> MEVHDFETDEFNDFNEDDYATREFLNPDERMTYLNHADYNLNSPLISDDIDNLIRKFNSLPIPSMWDSKNWDGVLEMLTSCQANPISTSQMHKWMGSWLMSDNHDASQGYSFLHEVDKEAEITFDVVETFIRGWGNKPIEYIKKERWTDSFKILAYLCQKFLDLHKLTLILNAVSEVELLNLARTFKGKVRRSSHGTNICRIRVPSLGPTFISEGWAYFKKLDILMDRNFLLMVKDVIIGRMQTVLSMVCRIDNLFSEQDIFSLLNIYRIGDKIVERQGNFSYDLIKMVEPICNLKLMKLARESRPLVPQFPHFENHIKTSVDEGAKIDRGIRFLHDQIMSVKTVDLTLVIYGSFRHWGHPFIDYYTGLEKLHSQVTMKKDIDVSYAKALASDLARIVLFQQFNDHKKWFVNGDLLPHDHPFKSHVKENTWPTAAQVQDFGDKWHELPLIKCFEIPDLLDPSIIYSDKSHSMNRSEVLKHVRMNPNTPIPSKKVLQTMLDTKATNWKEFLKEIDEKGLDDDDLIIGLKGKERELKLAGRFFSLMSWKLREYFVITEYLIKTHFVPMFKGLTMADDLTAVIKKMLDSSSGQGLKSYEAICIANHIDYEKWNNHQRKLSNGPVFRVMGQFLGYPSLIERTHEFFEKSLIYYNGRPDLMRVHNNTLINSTSQRVCWQGQEGGLEGLRQKGWTILNLLVIQREAKIRNTAVKVLAQGDNQVICTQYKTKKSRNVVELQGALNQMVSNNEKIMTAIKIGTGKLGLLINDDETMQSADYLNYGKIPIFRGVIRGLETKRWSRVTCVTNDQIPTCANIMSSVSTNALTVAHFAENPINAMIQYNYFGTFARLLLMMHDPALRQSLYEVQDKIPGLHSSTFKYAMLYLDPSIGGVSGMSLSRFLIRAFPDPVTESLSFWRFIHVHARSEHLKEMSAVFGNPEIAKFRITHIDKLVEDPTSLNIAMGMSPANLLKTEVKKCLIESRQTIRNQVIKDATIYLYHEEDRLRSFLWSINPLFPRFLSEFKSGTFLGVADGLISLFQNSRTIRNSFKKKYHRELDDLIVRSEVSSLTHLGKLHLRRGSCKMWTCSATHADTLRYKSWGRTVIGTTVPHPLEMLGPQHRKETPCAPCNTSGFNYVSVHCPDGIHDVFSSRGPLPAYLGSKTSESTSILQPWERESKVPLIKRATRLRDAISWFVEPDSKLAMTILSNIHSLTGEEWTKRQHGFKRTGSALHRFSTSRMSHGGFASQSTAALTRLMATTDTMRDLGDQNFDFLFQATLLYAQITTTVARDGWITSCTDHYHIACKSCLRPIEEITLDSSMDYTPPDVSHVLKTWRNGEGSWGQEIKQIYPLEGNWKNLAPAEQSYQVGRCIGFLYGDLAYRKSTHAEDSSLFPLSIQGRIRGRGFLKGLLDGLMRASCCQVIHRRSLAHLKRPANAVYGGLIYLIDKLSVSPPFLSLTRSGPIRDELETIPHKIPTSYPTSNRDMGVIVRNYFKYQCRLIEKGKYRSHYSQLWLFSDVLSIDFIGPFSISTTLLQILYKPFLSGKDKNELRELANLSSLLRSGEGWEDIHVKFFTKDILLCPEEIRHACKFGIAKDNNKDMSYPPWGRESRGTITTIPVYYTTTPYPKMLEMPPRIQNPLLSGIRLGQLPTGAHYKIRSILHGMGIHYRDFLSCGDGSGGMTAALLRENVHSRGIFNSLLELSGSVMRGASPEPPSALETLGGDKSRCVNGETCWEYPSDLCDPRTWDYFLRLKAGLGLQIDLIVMDMEVRDSSTSLKIETNVRNYVHRILDEQGVLIYKTYGTYICESEKNAVTILGPMFKTVDLVQTEFSS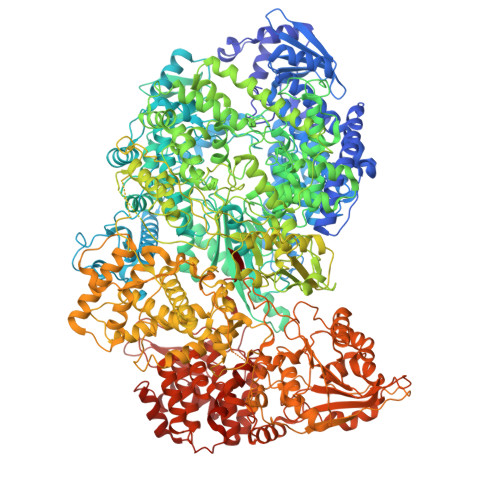SQTSEVYMVCKGLKKLIDEPNPDWSSINESWKNLYAFQSSEQEFARAKKVSTYFTLTGIPSQFIPDPFVNIETMLQIFGVPTGVSHAAALKSSDRPADLLTISLFYMAIISYYNINHIRVGPIPPNPPSDGIAQNVGIAITGISFWLSLMEKDIPLYQQCLAVIQQSFPIRWEAVSVKGGYKQKWSTRGDGLPKDTRISDSLAPIGNWIRSLELVRNQVRLNPFNEILFNQLCRTVDNHLKWSNLRRNTGMIEWINRRISKEDRSILMLKSDLHEENSWRD> GPLGSSWAPSDLAERAEAMTLSDCQQELSLVQTVTRGSRAFLSREEAQHFVKECGLLNCE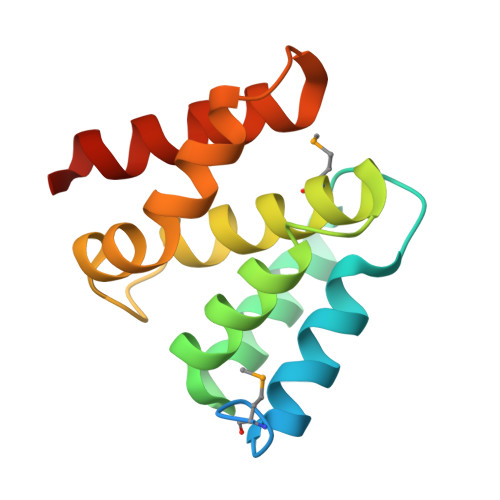AVLELLICHLGGTSECVQMRALGAVASLGCTDLLPQEHILLLTRPRLQELSAGSPGPVTNKATKILRHFEASCRQRP>MSEEQKTISISELESMNIKQLYEIAKSLGIPRYTSMRKRDLIFAILKAQTESTGYFFGEGVLEIHPEGFGFLRRIEDNLLPSNDDIYISPSQIRKFNLNTGDIISGVIRKPKEGEKYFAMIKIEAINYRPVEAVNDRVNFDNLTPDYPRERFILETDPKIYSTRLIDLFAP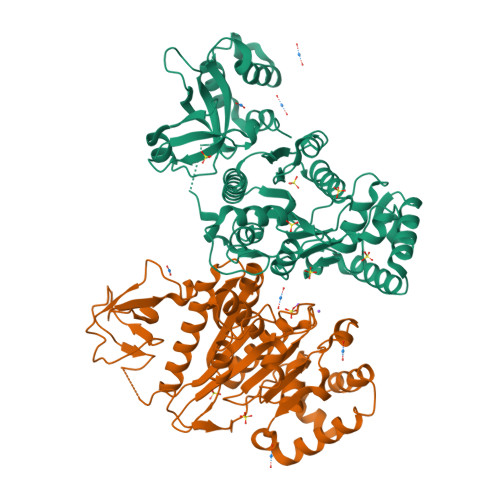IGKGQRGMIVAPPKAGKTTILKEIANGIAENHPDTIRIILLIDERPEEVTDIRESTNAIVIAAPFDMPPDKQVKVAELTLEMAKRLVEFNYDVVILLDSLTRLARVYNIVVPPSGKLLTGGVDPAALYKPKRFFGAARNTREGGSLTIIATALVETGSKMDEVIFEEFKGTGNMELVLSRQLANKRIFPAINLLLSGTRREELLLDEETLKKVWLLRRMLSAMTEEEGLTLILNKLSETSSNEEFLKLIDKEKARY[2x]The RADAR system comprises two genes, rdrA that encodes a protein with an ATPase domain, and rdrB, encoding a predicted adenosine deaminase domain protein. Here, we determine cryo-EM structures of the RADAR defense complex, revealing RdrA as a heptameric, two-layered AAA+ ATPase and RdrB as a dodecameric, hollow complex with twelve surface-exposed deaminase active sites. RdrA and RdrB join to form a giant assembly up to 10 MDa, with RdrA docked as a funnel over the RdrB active site. Our results define ATP mononucleotide deamination as a determinant of RADAR immunity and reveal supramolecular assembly of a nucleotide-modifying machine as a mechanism of anti-phage defense.

We analyzed mixed samples of purified E. coli RdrA and RdrB by negative-stain EM and observed gigantic flower-like arrangements with a central hub surrounded by up to six “petals”. Further analysis with cryo-EM confirmed specific RdrA-RdrB co-complex formation and allowed us to determine a 6.7 Å structure of a representative single-petal complex. In the RdrA-RdrB complex, RdrA is positioned such that the central heptameric channel funnels directly into the catalytic core of RdrB. In agreement with negative-stain EM analysis of multi-petal complexes, the RdrA heptamer footprint sits primarily over a single RdrB protomer and leaves room for a total of 12 docked RdrA complexes on the RdrB core dodecameric shell. Nearly all contacts between RdrA and RdrB are mediated by residues that reside in an RdrA α-helical insertion that forms a crown on top of the AAA+ ATPase domain. We introduced several mutations predicted to disrupt the formation of the RdrA-RdrB complex, including charge-swap mutations of conserved residues in the RdrA crown (K150E, E151K, and R162E) and observed that mutations to residues involved in RdrA-RdrB complex formation significantly decrease or ablate RADAR defense. Modeling of a complete ∼10 MDa flower-like RdrA-RdrB complex demonstrates that the RdrB adenosine deaminase active site remains solvent-accessible, suggesting that supramolecular assembly could represent that active state of the RADAR defense complex. Instead, we observed that the addition of RdrA to RdrB leads to enhanced conversion of ATP to ITP supporting that activation of RdrA in vivo likely leads to induction of RdrB activity.

>MERFLLNSTVLLYRLSTVSLDEVSLDERVESSVFLAQYEQARSLPDHVAKSAWSYLVQQIKQRNMKLGPVAILRLIAEKFIKNEKGGPKIDLPMFSEWQTLMSRVSCLPIIACHQVFNPGPASQEYSFRWPLYPYHPTVEDYITRECLHETHQHLNGSTSAEECWLDALKHPEACLRDFEKGWASQEMKQLCAQIDPSLTPRIFKDRLQIACNIREILCRVAQGVELPEWIASMQNPQQLANSTILHNGREYGFATVWPIDDKYSQESEFCWLTGLLEKWRFNAPEGLERLLWIYLLIQNQYLTLLVQRDDFFGFEQFQNYTMTELREETEKSYLSRFKHAHGAGVYSQVRYLEGRFAPKSDPNKMQKLLFSVLRGYWEYLSAHMSMEWVHEKPLTISQVLDNLELVEPHGKCVELALVPHFIKRKPKNGEAYPHALLFKDLKNQAAILMDMLKSEPRLTGWIRGVDAAANEMHAPPELFCPLFRVLAKSGIAHFTYHVGEDFPHLISGIRSIDDALRFLPLRNGDRLGHCTAIGITPSIWKRSLPLSLSMTKETRLLDLVFIWRELRSHPELLRYASDAAIEAVRLAHKVFSLEEEVSITTLDQVFEMRGLLAESEGLLSELNEPLKPKSLWLEEYERARELVKTTGMKRPLKLYKQWLTSDNVRKQRAEYVEVALEYLPDEAVVALQQAVMAKMADRNIAIECPPTSNTRISQYRNVSEHHIFRWMGLPGEAIEGDVPMSICLGSDDPGIFAADLKSEFYHLFVVLTRKFGLSPADALRKVAEVNENGRIYRFHDVS[12x];>[7x]MTDSVQTETTKGKIIINLFAPNLSGSTKEDDLIQKSLRDQLVESIRNSIAYPDTDKFAGLTRFIDEPGRNVFFVDGTRGAGKTTFINSVVKSLNSDQDDVKVNIKCLPTIDPTKLPRHEPILVTVTARLNKMVSDKLKGYWASNDYRKQKEQWQNHLAQLQRGLHLLTDKEYKPEYFSDALKLDAQLDYSIGGQDLSEIFEELVKRACEILDCKAILITFDDIDTQFDAGWDVLESIRKFFNSRKLVVVATGDLRLYSQLIRGKQYENYSKTLLEQEKESVRLAERGYMVEHLEQQYLLKLFPVQKRIQLKTMLQLVGEKGKAGKEEIKVKTEPSMQDIDAIDVRQAIGDAVREGLNLREGSDADMYVNELLKQPVRLLMQVLQDFYTKKYHATSVKLDGKQSRNERPDELSVPNLLRNALYGSMLSNIYRAGLNYEQHRFGMDSLCKDIFTYVKQDRDFNTGFYLRPQSESEALRNCSIYLASQVSENCQGSLSKFLQMLLVGCGSVSIFNQFVTELARAENDREKFEQLISEYVAYMSVGRIESASHWANRCCAVVANSPNDEKIGVFLGMVQLNRKSRQNMPEGYKKFNIDTENGLAKAAMASSLSTVASNNLMDFCSVFNLIGAIADISACRCERSAITNAFNKVIAQTTCIVPPWSEAAVRAEMKGSSKSADNDAAVLDVDLDPKDDGVIDESQQDDATEFSDAITKVEQWLKNVNEIEIGIRPSALLIGKVWSRFYFNLNNVADQHKTRLYRNAEHGRMASQSNAAKIMRFNVLAFLHAVLVEESLYHSVSDREYIGEGLRLNPVTSVDEFEKKIKIIGEKLKADNKTWKNTHPLFFLLISCPILHPFIFPIGGINCSVKALNKETSFNKLIDEIVGDKLLSDEEWDYLTKNNDQKTNTRQQIFQNTITSLNSSTIVGASYDKDTPARKTKSPSLGDSEEK> MSAEKLFTPLKVGAVTAPNRVFMAPLTRLRSIEPGDIPTPLMGEYYRQRASAGLIISEATQISAQAKGYAGAPGLHSPEQIAAWKKITAGVHAEDGRIAVQLWHTGRISHSSIQPGGQ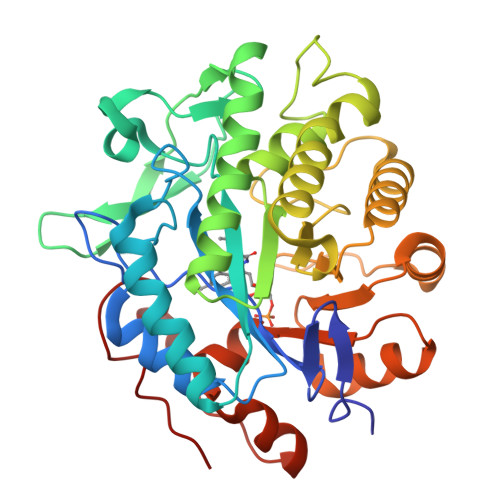APVSASALNANTRTSLRDENGNAIRVDTTTPRALELDEIPGIVNDFRQAVANAREAGFDLVELHSAHGYLLHQFLSPSSNQRTDQYGGSVENRARLVLEVVDAVCNEWSADRIGIRVSPIGTFQNVDNGPNEEADALYLIEELAKRGIAYLHMSETDLAGGKPYSEAFRQKVRERFHGVIIGAGAYTAEKAEDLIGKGLIDAVAFGRDYIANPDLVARLQKKAELNPQRPESFAGGGAEGYTDYPSL>MFPKNFKFGFSEAGFQFEMGVSDIDTNTDWYKWSHDSENIKNHIVSGDRPEEGVGYWDLYPKDHDLAEYIGMNAARIGIEWSRIFPVSTERVTVEVIEENGDILEIKITEKTIKELDLLSDKNAMQHYTNIFNDIKKRGWFLVINLFHWSLPLWINDPSNRNSEKDNALGNCMNRSSVIEFVKYAAYISYYFGSIADRFATMNEPNEVFKTCSEDKRVESYHIRMKWFVEAHARSYDAMKQFTNRQIGVIYANGDVQSFENKDPKLKEEVEYEQRYSFFDALIHGDVHWYVGACRKTNHVHGKSIRPDLSNRIDWIGVNYYSRNVVKRKEDGYENVRGLGYDTGWVSYEKSLDGRSVSETGWEIYPEGIYNIVMSYHKRYELPMMITENGMADDNDRFRPRYLVSHLKNLERAINDGAKVDGYLHWALTDNFEWGSGFSKKFGLIKVDYKTKKRYLRPSALIMKEIT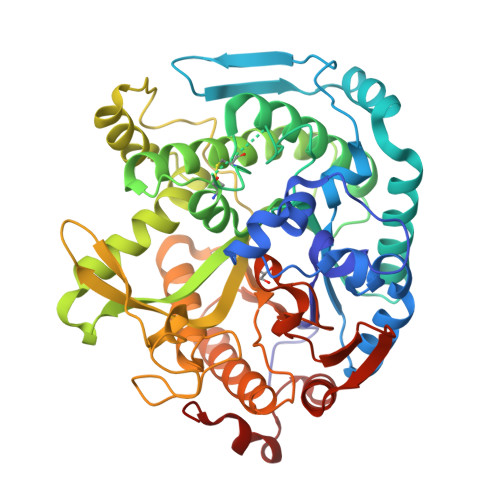KHNGIPEELEWLGEDKF[2x]>[4x]MAPTRRSRDLLRGKNVLIIGGTSGIGFAVAQLVIEHGAMACIAGSNPTKLGKALDALKQHPDRDPIAIVQSATCDLFDVPNLEQNLDNLLKLAAGDSKIHHIVFTAADMV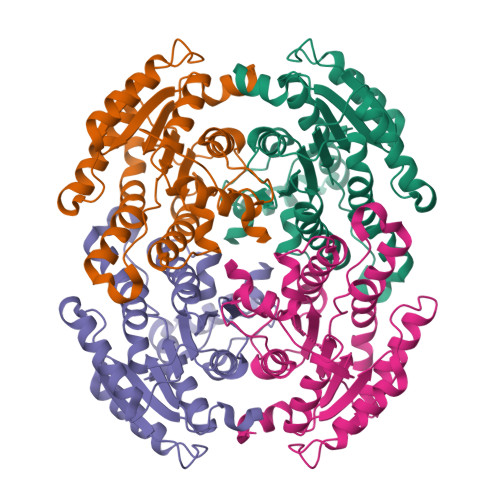QPPPLASVTIEQIQRVGTIRFTAPMLVAKLLPKYMELCPENSYTLTSGSHAKQPDPGWSLVTGYCGGVEGLMRGLAVDMMPLRVNVVSPGAVLTPVLRDILGDSLEIALDAARKKSTTGRIARPEDVAEAYLYIMKDQNITGTVLETSAGMLLR1-((2R,3R,4S,5R)-TETRAHYDRO-3,4-DIHYDROXY-5-(HYDROXYMETHYL)FURAN-2-YL)PYRIDINE-2,4(1H,3H)-DIONE | C10 H13 N O6 | 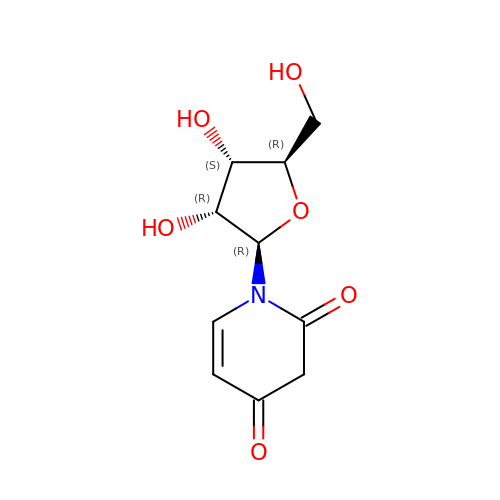WIRVQQCUKDPURA-PEBGCTIMSA-N> GSASPAVAELCQNTPETFLEASKLLLTYADAILRNPNDEAARSIRIGNTAFSTRLLPVRGAVECLFEMGFEEGETHLIFPKKASVEQLQKIRDL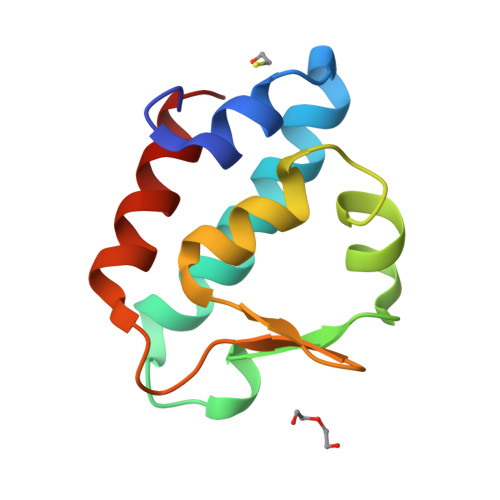IAIER>MTNTDLKPLLDNLRNATEFWNLVAAASATDESTVHNRSYRDALDWLESAALALGDALIAQRKAVG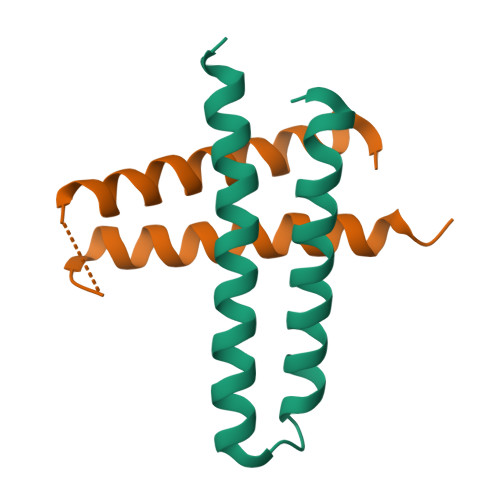GDHE[2x]>MVKVTYDIPTCEDYCALRINAGMSPKTREAA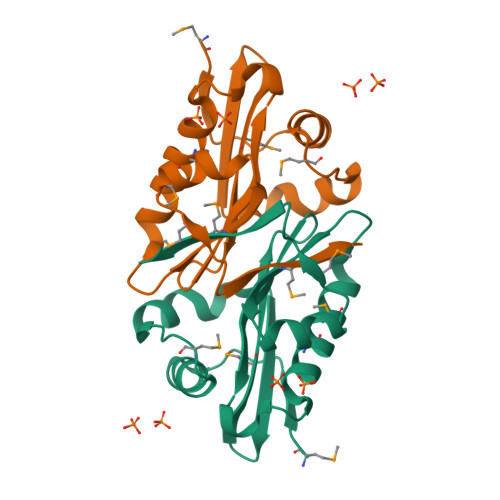EKGLPNALFTVTLYDKDRLIGMGRVIGDGGTVFQIVDIAVLKSYQGQAYGSLIMEHIMKYIKNVSVESVYVSLIADYPADKLYVKFGFMPTEPDSGGMYIKY[2x]>[2x]GSPLPSDVRPPHILVKTLDYIVDNLLTTLPESEGFLWDRMRSIRQDFTYQNYSGPEAVDCNERIVRIHLLILHIMVKSNVEFSLQQELEQLHKSLITLSEIYDDVRSSGGTCPNEAEFRAYALLSKIRDPQYDENIQRLPKHIFQDKLVQMALCFRRVISNSAYTERGFVKTENCLN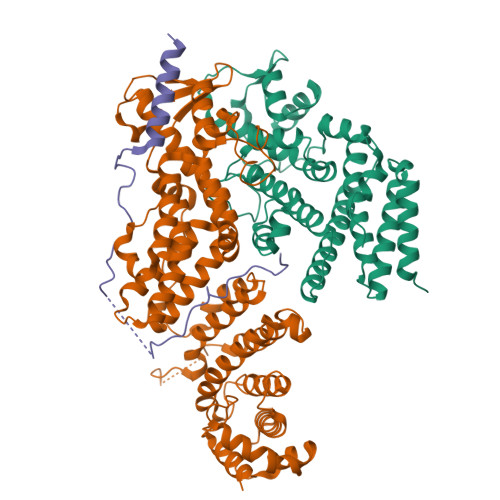FYARFFQLMQSPSLPLLMGFFLQMHLTDIRFYALRALSHTLNKKHKPIPFIYLENMLLFNNRQEIIEFCNYYSIEIINGDAADLKTLQHYSHKLSETQPLKKTYLTCLERRLQKTTYKGLINGGEDNLASSVYVKDPKK;>MDMANQLLDELAHGNFSHLTLNLSQNGREIAILQKQLTGFDDKQLETFVEQHPAMPNDTRFKIMCTSFLNYARDVDPWSAWSSSDLIFEFYQCLINCLINDNAPHIEMLIPVATRETEFIINLAGKLDSFHLQLHTRSHQFLSHISSILSRLFNSIKPPRGNASSTNIPGKQRILLYLVNKLNNIYFRIESPQLCSNIFKNFQPKSMLAHFNEYQLDQQIEYRYLLGRYYLLNSQVHNAFVQFNEAFQSLLNLPLTNQAITRNGTRILNYMIPTGLILGKMVKWGPLRPFLSQETIDNWSVLYKHVRYGNIQGVSLWLRQNERHLCARQLLIVLLEKLPMVTYRNLIKTVIKSWTTEWGQNKLPYSLIERVLQLSIGPTFEDPGAQEITIYNGIHSPKNVENVLVTLINLGLLRANCFPQLQLCVVKKTTMIQEIVPPVNERITKMFPAHSHVLW[2x];>[2x]MSTDVAAAQAQSKIDLTKKKNEEINKKSLEEDDEFEDFPIDTWANGETIKSNAVTQTNIWEENWDDVEVDDDFTNELKAELDRYKRENQ2-ANHYDRO-3-FLUORO-QUINIC ACID | C7 H9 F O5 | 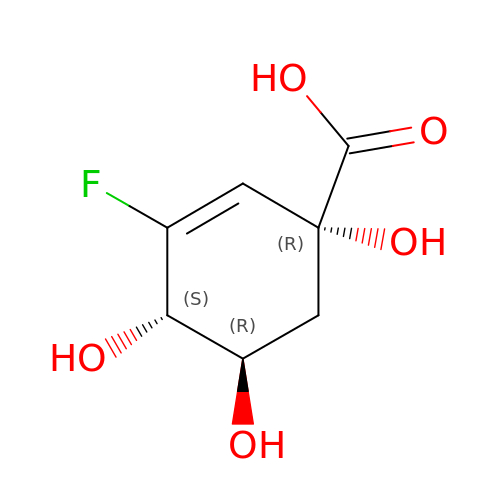DGZQZSSRYAJDAX-XAHCXIQSSA-N> SDEAFKMPASRYLTDMTIEEMSRDWFMLMPKQKVAGPLCVRMDQAIMDKNIILKANFSVIFDRLETLTLLRAFTEEGAIVGEISPLPSLPGHTNEDVKNAIGVLIGGLEWNDNTVRVSETLQRFAWRSSNEN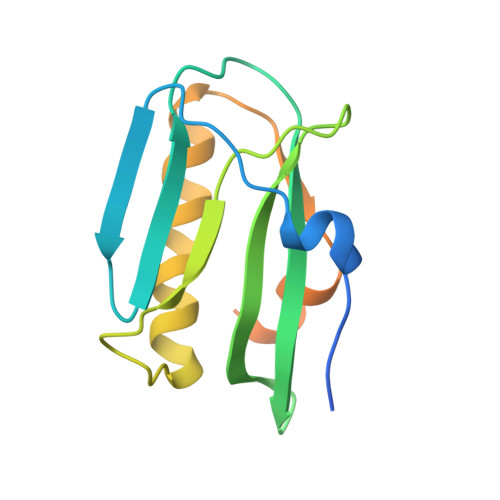GGPPLTPTQKRKMAGTIRSEV> MGSSHHHHHHSQDPKPRVLVLTGAGISAESGIRTFRAADGLWEEHRVEDVGTPEGFDRDPELVQAFYNARRRQLQQPEIQPNAAHLALAKLQDALGDRFLLVTQNCDNLHERAGNTNVIHMHGELLKVRCSQSGQALDWTGDVTPEDKCHCCQFPAPLRPHVVWFGEMPLGMDEIYMALSMADIFIAIGTSGHVYPAAGFVHEAKLHGAHTVELNLEPSQVGNE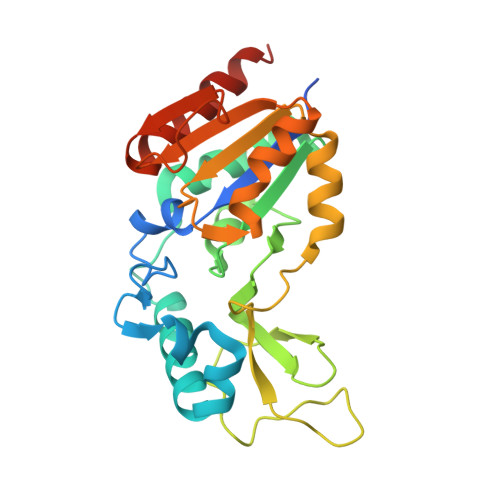FAEKYYGPASQVVPEFVEKLLKGLKAGSIA In the major clinical pathogen Pseudomonas aeruginosa, PBP1B is anchored within the cytoplasmic membrane but regulated by a bespoke outer membrane-localized lipoprotein known as LpoP. Here, we report the structure of LpoP, showing an extended N-terminal, flexible tether followed by a well-ordered C-terminal tandem-tetratricopeptide repeat domain. We show that LpoP stimulates both PBP1B transpeptidase and glycosyltransferase activities in vitro and interacts directly via its C terminus globular domain with the central UB2H domain of PBP1B. LpoP is a predicted lipoprotein of 259 amino acids with a clear lipobox signal sequence that promotes localization and attachment to the P. aeruginosa outer membrane via an N-terminal lipid modification at Cys19 (Greene et al., 2018).

Crystals of P. aeruginosa LpoP143-259 displayed monoclinic P21 symmetry with unit cell dimensions of a = 48.8 Å, b = 154.6 Å, c = 54.1 Å, and β = 90.1°, and diffracted with a resolution of 2.2 Å. There are eight molecules of LpoP in the asymmetric unit. The resulting maps showed well-resolved electron density for most of the protein chain, allowing near complete tracing of the ordered part from residues 152 onward (see the STAR Methods). The structure indicated a monomeric form of the protein with no obvious crystallographic formation of larger oligomers. LpoP143-259 is made up of six α helices (H1–H6) of variable length that form helix-turn-helix motifs similar to those of TPRs and that are linked together through short loops (Cortajarena et al., 2004, Zeytuni and Zarivach, 2012). Numerous inter-helical hydrophobic contacts favored by the high percentage of Leu (12%) and Ala (22%) stabilize the core structure. LpoP has a striking structural similarity to protein domains formed by repetition of TPR domains (prosite PS50293 family). LpoP's C-terminal globular domain exclusively consists of three repeated TPR motifs, giving it primarily alpha-helical character and a structure greatly similar to the N-terminal domain of CpoB. The maximal chemical shift perturbations were mapped on the LpoP structure and found to concentrate mainly in the region connecting the extremities of helix 2 and helix 3. This region also contains the most conserved amino acid residues as obtained by alignment of 150 sequences using ConSurf software.

>SAGSLAADEQLDGPVLAMLTTAQQQQGSGDLNSAAASLERAQRIAPREPQVLYRLAQVRLAQGDAAQAEQVARRGLSYANGRPALQAGLWELIAQAREKQGDSAGAALARQKAKVS[8x]>[2x]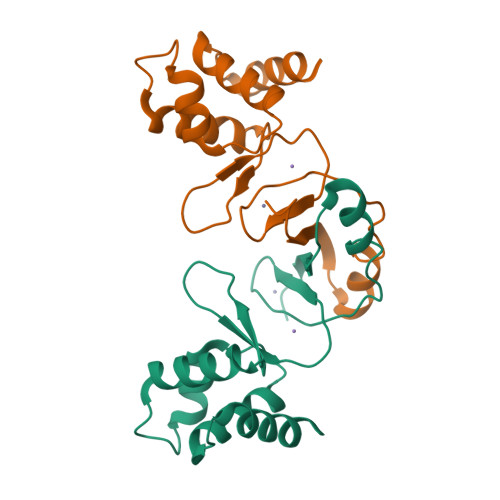MAAHELKEALETLKETGVRITPQRHAILEYLVNSMAHPTADDIYKALEGKFPNMSVATVYNNLRVFRESGLVKELTYGDASSRFDFVTSDHYHAICENCGKIVDFHYPGLDEVEQLAAHVTGFKVSHHRLEIYGVCQECSKKENH PHOSPHORIC ACID 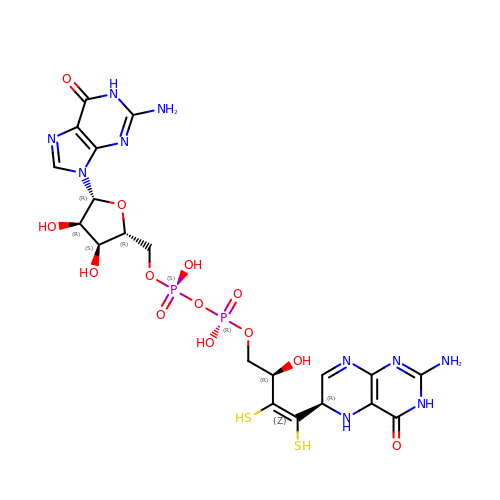4-(2-AMINO-4-OXO-3,4,5,6,-TETRAHYDRO-PTERIDIN-6-YL)-2-HYDROXY-3,4-DIMERCAPTO-BUT-3-EN-YL ESTER GUANYLATE ESTER | C20 H26 N10 O13 P2 S2 | IRGDLSAXQOKWLX-XHEYTWMPSA-N> SNAMREIVWVHSQRIAPYKTLILNEFCYYPLELDPTPFNALIFTSKN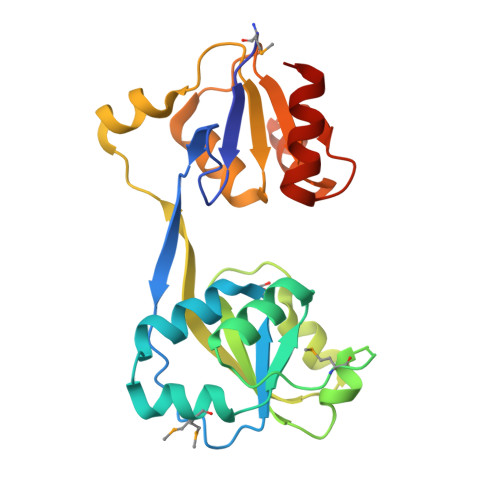AVFSLLETLKNSPKLKMLQNIPAYALSEPTAKTLQDHHFKVAFMGEKAHGKEFVQEIFPLLEKKSVLYLRAKEIVSSLDTILLEHGIDFKQAVVYENKLKHLTLSEQNALKPKEKSILIFTAISHAKAFLHYFEFLENYTAISIGNTTALYLQEQGIPSYIAKKPSLEACLELALSLRIKEC Immunoglobulin E (IgE) is a central regulatory and triggering molecule of allergic immune responses. IgE’s interaction with CD23 modulates both IgE production and functional activities.CD23 is a noncanonical immunoglobulin receptor, unrelated to receptors of other antibody isotypes. Human CD23 is a calcium‐dependent (C‐type) lectin‐like domain that has apparently lost its carbohydrate‐binding capability. The calcium‐binding site classically required for carbohydrate binding in C‐type lectins is absent in human CD23 but is present in the murine molecule.

To determine whether the absence of this calcium‐binding site affects the structure and function of human CD23, CD23 mutant proteins with increasingly “murine‐like” sequences were generated. Restoration of the calcium‐binding site was confirmed by NMR spectroscopy, and structures of mutant human CD23 proteins were determined by X‐ray crystallography, although no electron density for calcium was observed. This study offers insights into the evolutionary differences between murine and human CD23 and some of the functional differences between CD23 in different species.

> SGFVCNTCPEKWINFQRKCYYFGKGTKQWVHARYACDDMEGQLVSIHSPEEQDFLTKHASHTGSWIGLRDLDLEGEFIWVDGSHVDYSNWAPGEPNNRSQGEDCVMMRGSGRWNDAFCDRKLGAWVCDRLATCTPPASEGSAE>[2x]SNAEQYHSQVVGKIGYIARCMQTIDPENNLKKIREDYQDVLIWAEKNYRFEEILEASKSGKCPNDLDALSRRSLILQELLRLVSSISPFKMKLDLIESQYEKMKQHVNLWKSDYHVKLNQLNQLTDYLKNAAPTPKNNFLRAMTSVLQMQIAQYGITEDNEGINQLFKLGLHLLAMANEKIDEQYHLFKGYVKDQPEESPFEGILPAEDQKILVKTMIDYAMPKLSSKVLQDKLSALSSSDVLTKTLLDSIDRIVKENEKLNALSK

The protein SidK, secreted by Legionella pneumophila, interacts with the V-ATPase to inhibit acidification of the phagolysosome in the early stages of infection. V-ATPases pump protons across a phospholipid membrane using energy from the hydrolysis of adenosine triphosphate (ATP) to adenosine diphosphate (ADP) and inorganic phosphate. Successful pathogens can subvert host defenses by secreting effectors that target V-ATPases to inhibit lysosomal acidification or lysosomal fusion with other cell compartments. This study reveals the structure of the V-ATPase:SidK complex, an assembly formed from the interaction of host and pathogen proteins involved in the infection of phagocytic white blood cells by Legionella pneumophila. Removal of the C-terminal residues 415–573 of SidK did not significantly affect V-ATPase inhibition by the SidK mutants, but truncations of the N-terminal region of the protein has been demonstrated to prevent V-ATPase inhibition. These data show that binding of the N-terminal domain of SidK to the V-ATPase is responsible for its partial yet specific inhibition of V-ATPase activity.

One SidK construct, consisting of residues 16–278 (SidK-N), yielded two crystal forms that diffracted X-rays to 2.3 to 2.4 Å resolution and the structure of SidK-N was determined from these crystals. The second crystal form of SidK(16–278) contained two molecules in the asymmetric unit related by a non-crystallographic two-fold symmetry. In this crystal form SidK-N exists as a dimer, with the two molecules swapping their second and third α-helical bundles (red arrowheads and oval). This domain swapping is accomplished by a rotation of ~180° relative to the first α-helical bundle that occurs through conformational changes within the short linker connecting the first and second α-helical bundles (residues 117–125). The domain swapping retains the interface between the first and second α-helical bundles seen in the first crystal form and the domain-swapped monomer is similar to the monomer in the first crystal form. The monomeric SidK predominates in solution, even at high concentrations, and therefore the elongated monomer structure is expected to be the functional state of the protein. The flexibility between the first and second α-helical bundles is consistent with the flexibility in the linker between these bundles observed by X-ray crystallography.>MSAHRTLLLRLSDSGEPVTSCSYGQGVLTLPSLPLPQGKKLGDMPVYTVKLAIPAGSPVTRDGLIWTNCPPDFSTQFDREKFYKKIIKTSFHEDDHIDLDIYVPGTYCFYLSFKNDKDELETTRKFYFVVLPILSVNDKFIPLNSIAMQSVVSKWMGPTIKDWEKVFARVASKKYNMIHFTPLQHRGESNSPYSIYDQLEFDPTVFKSEKEVADMVERLRTEHNILSLTDIVFNHTANNSQWLLDHPEAGYNHKTSPHLISAIELDKKLLDFSEQMEALGYPVDLKTVDDLIKVMDGIKEHVIGELKLWEFYVVDVKQTVSELREKWGN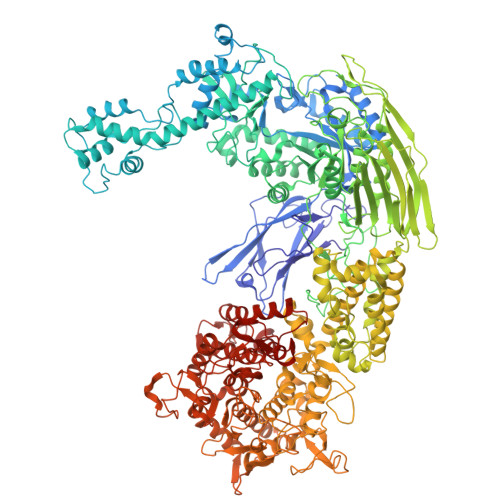SKSWSDDNIPSKDDSTNLAQFVRDNATEPGFGSLGERGSNKINIDKFAAILKKLHSEDYNNGIEELATKILNDINLPFYKEYDDDINEVLEQLFNRIKYLRIDDHGPKQGPITKKLPLSEPYFTRFKAKDGEEYALANNGWIWDGNPLVDFASSQSKAYLRREVIVWGDCVKLRYGKGPSDSPYLWERMSKYVEMNARIFNGFRIDNCHSTPLHVGQYFLDVARRVNPNLYVVAELFSGSEAMDCLFVERLGISSLIREAMQAWSEEELSRLVHRHGGRPIGSYKFVPLDDFPYPADVKIDEEYCAYNPDDHSVKCVSEIMIPKTLTATPPHALFMDCTHDNETPNQKRTVEDTLPNAALVAFCSSAIGSVYGYDEVFPQLLDLVQEKRTYSCAENTGISKVKTLLNNMREEIASEAVDIEDSEMHVHHDGQYITFHRTNAKNGKGWYLVARTKFHSSGDQMLPRIKLSQTKATFKAAFSLERTGDAPISDEIIEGIPTKLRELTGFDIGFDENTKETSILLPQDFPQGSIVIFETQQLGIDDSLDHFIRSGAIKATEKLSLESINYVLYRAEQEEYDYSEGRSGAYDIPDYGKPVYCGLQGWVSILRKIIFYNDLAHPLSNNLRNGHWAVDYVVNRLDLYKDKEGVAEVQEWLRSRMERIKQLPSYLVPSFFALVVGIMYGCCRLRAMQLMSDNVGKSTVFVQSLAMTSIQMVSAMKSTSILPDQNIAAMAAGLPHFSTNYMRCWGRDVFISLRGLLLTTGRYEEAKEHILAFAKTLKHGLIPNLLDAGRNPRYNARDAAWFFVQAIQDYVTIVPGGVSLLQEKVTRRFPLDDEYIPYDDPKAFSYSSTIEEIIYEILNRHAGGIKYREANAGPNLDRVMKDEGFNVEVNVDWETGLIHGGSQFNCGTWMDKMGESEKANSVGVPGTPRDGAAVEINGLLKSCLRFVLQLSKDGKFKYTEVTKPDGSKISLSSWNDLLQENFERCFYVPKNKEDDNKFEIDATIINRRGIYKDLYRSGKPYEDYQFRPNFTIAMVVAPELFTPDYAAGAIELADQVLRGPVGMRTLDPSDYNYRPYYNNGEDSDDFATSKGRNYHQGPEWVWCYGYFIRAYHYFNFLTNPKCQVEGSAKKLKPSSYLYRKLYSRLLKHREWIENSPWAGLAELTNKDGEVCNDSSPTQAWSTGCLLDLFYDLWISYEE[2x]> VHNDVTVPDFSAYRREDVMDATTSSQTSSEDRKGFSYLVTATACVATAYAAKNVVTQFISSLSASADVLALSKIEIKLSDIPEGKNVAFKWRGKPLFVRHRTQAEINQEAEVDVSKLRDPQHDLDRVKKPEWVILVGVCTHLGCVPIANSGDFGGYYCPCHGSHYDA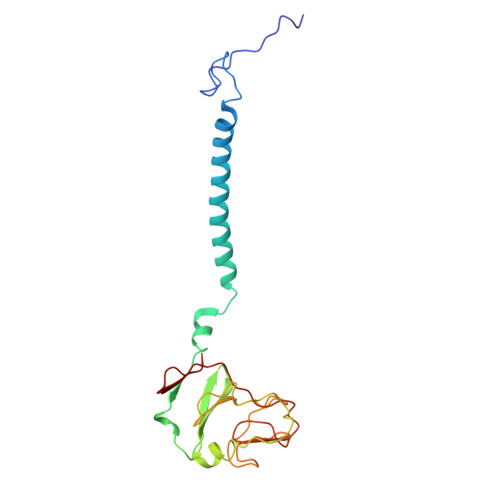SGRIRKGPAPYNLEVPTYQFVGDDLVVVG> MVIIKLNANKNMPVLAVEKPQEIHKEELSDHHQSNGFTS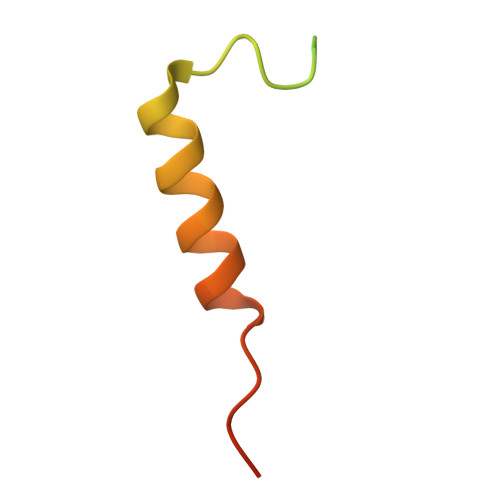LDLEMIELENFVLHCPLPEENLAG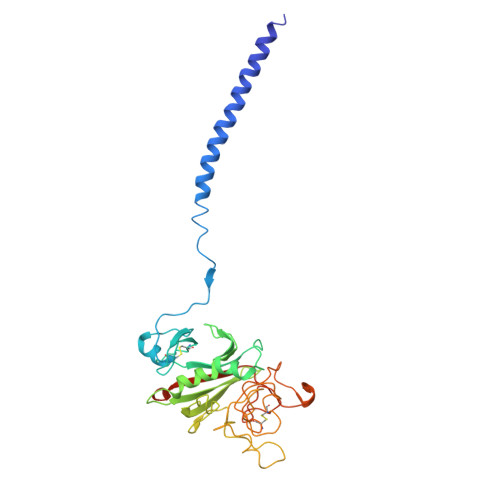> KMLEEIMKYEASILTHDSSIRYLQEIYNSNNQKIVNLKEKVAQLEAQCQEPCKDTVQIHDITGKDCQDIANKGAKQSGLYFIKPLKANQQFLVYCEIDGSGNGWTVFQKRLDGSVDFKKNWIQYKEGFGHLSPTGTTEFWLGNEKIHLISTQSAIPYALRVELEDWNGRTSTADYAMFKVGPEADKYRLTYAYFAGGDAGDAFDGFDFGDDPSDKFFTSHNGMQFSTWDNDNDKFEGNCAEQDGSGWWMNKCHAGHLNGVYYQGGTYSKASTPNGYDNGIIWATWKTRWYSMKKTTMKIIPFNRLTIGEGQQHHLGGAK> ETTQKLTVSHIEGYECQPIFLNVLEAIEPGVVCAGHDNNQP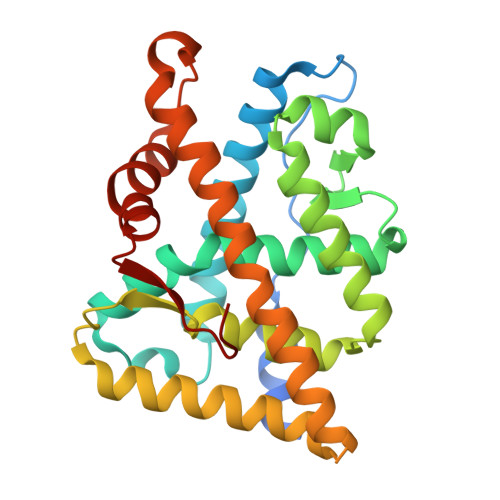DSFAALLSSLNELGERQLVHVVKWAKALPGFRNLHVDDQMAVIQYSWMGLMVFAMGWRSFTNVNSRMLYFAPDLVFNEYRMHKSRMYSQCVRMRHLSQEFGWLQITPQEFLCMKALLLFSIIPVDGLKNQKFFDELRMNYIKELDRIIACKRKNPTSCSRRFYQLTKLLDSVQPIARELHQFTFDLLIKSHMVSVDFPEMMAEIISVQVPKILSGKVKPIYFHTQ> HPETLVKVKDAEDQLGARVGYIELDLNSGKILESFRPEERFPMMSTFKVLLCGAVLSRVDAGQEQLGRRIHYSQNDLVEYSPVTEKHLTDGMTVRELCSAAITMSDNTAANLLLTTIGGPKELTAFLHNMGDHVTRLDRWEPELNEAIPNDERDTTMPAAMATTLRKLLTGELLTLASRQQLIDWMEADKVAGPLLRSALPAGWFIAD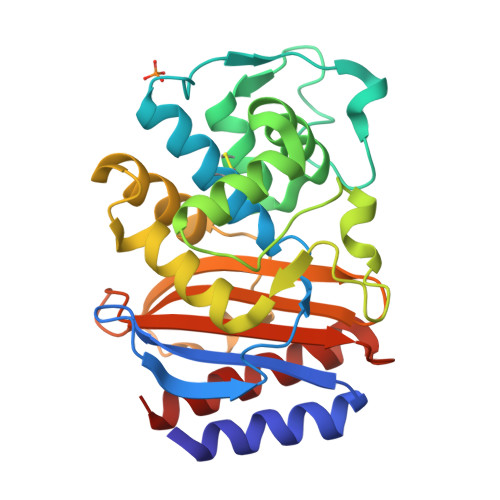KSGAGERGSSGIIAALGPDGKPSRIVVIYTTGSQATMDERNRQIAEIGASLIKHW>[2x]MSALDNSIRVEVKTEYIEQQSSPEDEKYLFSYTITIINLGEQAAKLETRHWIITDANGKTSEVQGAGVVGETPTIPPNTAYQYTS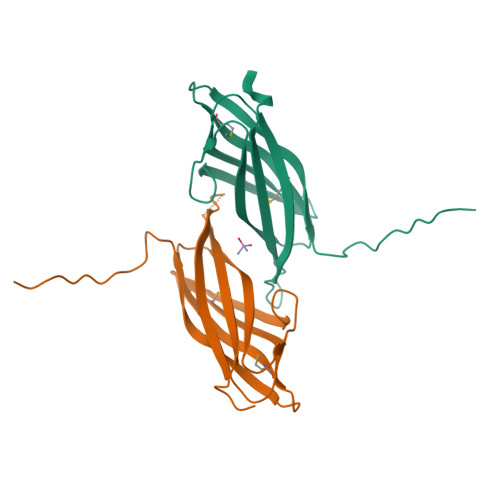GTVLDTPFGIMYGTYGMVSESGEHFNAIIKPFRLATPGLLHLEHHHHHH> MRRCVMAKGEDPAHVAGWDDRQDAVEWWWTEANDSRGRQRLEAAAAVAAAAASSTVGLPLFPRFSPGRRRRRRPPAPPPPPPPLFLSRHLHSMPWLWCTCVKMQMYYTPTALTCPLSNSLAAHVGHIIVGVAALLPYSMLLFLTVMCNPRKHEPVLRAQRIRWLTFHSLMFRLLRCITASPAVAASVAVAAAQTPTSLRPAAVCRRGVHLAPSVLAASAPPPPPQQQQQPTSAAVPASTATSTTTIAAGPYRRVGNVFIVTCIDHPFKFSWEVNRMLRELRLEFM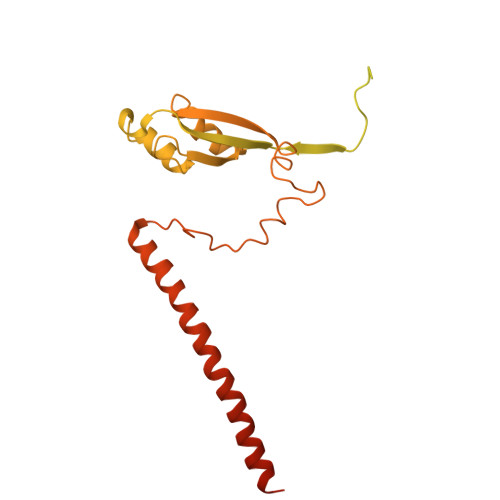GQTTVVPDIPPVRKRIWRVRHVVRVDQLDLDEAKALIGIPEHISFRDLAGQIPPTFGRGGSVANPHMRSKMNFMRLRRMRLRDVMHRDQLEKRLLEERHHALQQQQQQQQGGGEAAAAAAATTA> GS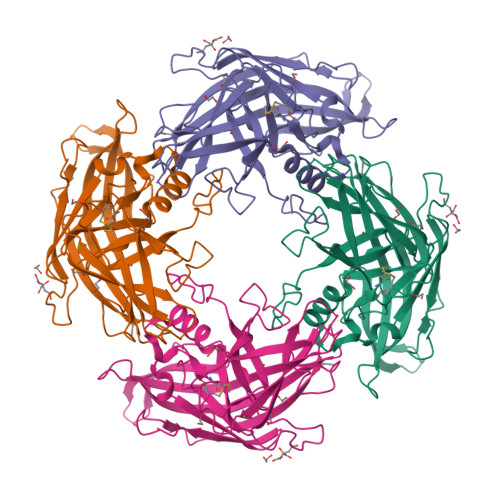EWEDEQYEHYISFSSQLDSKGVTNIYVPYSRHDAEGNYAEGGEGRSNYQLPILVSGSTDNPSNVTVHVAHDADTLNILNYARYATRTELYYEDMGAEGLAYASYPESLQIKAGENKGLLDLKFDFRNIDMSEKWVLPLQIVDDASYNYVAHPRKDYAKAILRIFPFNDYSGDYSGTGITNKVVTGYDGDGKPIETAESITKSSIRGYVIDEQTIFTYAGIVDEDYTDRRKYKIKFAFNGETNGSVTISCDNAEEIGFELNKDVTPSFRISSSMDDAKPYLEHRYVIINNVDYYFNYIPVEGTIIRYHVKGTLTLSRDINTQIPDEDQAIEW>[2x]SLSDKDKDSIKAFWAKISPKAEDIGADALARMLTVYPQTKTYFSHWKDLSPGSAPVKKHGKTVMGSVAEAVSKIDDLTNGLLTLSELHAFQ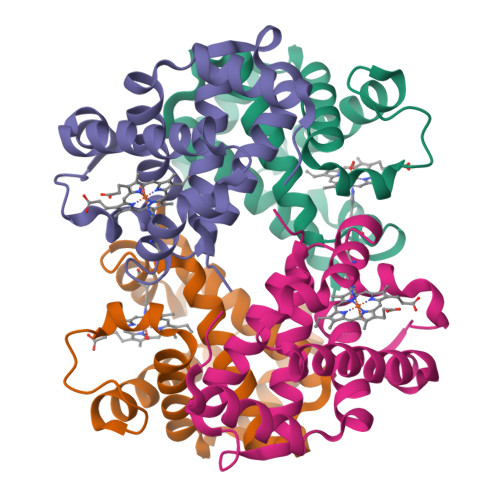LRVDPANFKILSHNLLVVLAQQFPNDFTPEVHVSMDKFLSLLSWSLSEKYR;>VEWSTAERSAIAGLWGKISVDEIGPQALSRLLIVYPWTQRHFAAFGNLSSPAAINGNPKVAHHGKVVMGGLERAIKNMDNIKAAYSSLSVMHSEKLHVDPDNFRLLADCITVCVAMKFGPSAFTPDVQEAWQKFLAVVVAALSRYH[2x]NA is a homotetrameric transmembrane glycoprotein responsible for cleavage of sialic acid from the host cell membrane. By blocking NA enzymatic activity, neuraminidase inhibitors (NAIs) prevent new viral particles from being released from the surface of an infected cell, thus stopping the spread of virus in the airways. In this study, we applied a set of experimental techniques using recombinant NA variants to understand the molecular basis of development of oseltamivir resistance in the viral N1 neuraminidase NA2009. To decipher the structural mechanism of resistance, we determined crystal structures of NA2009 mutants in complex with oseltamivir carboxylate.

Two variants (I223V and S247N single mutants) crystallized in the centered orthorhombic space group with two molecules in the asymmetric unit; the tetrameric biological unit could be reconstructed from two symmetrically related dimers. The I223V substitution did not induce any structural changes in the neighboring residues; however, the substitution for a smaller side chain results in enlargement of the volume of the enzyme active site pocket and loss of Van der Waals contacts with the pentyloxy substituent of oseltamivir. The methyl group of the I223 side chain in the wt enzyme forms a dispersion bond (C-C distance of 4.1 Å) with the methyl group of oseltamivir. This interaction is not present in the I223V mutant, where the closest C-C distance between V223 and oseltamivir methyl groups is 5.0 Å. The energy of this interaction can be estimated as ~1 kcal/mol. This explains the 30-fold increase in Ki value for oseltamivir upon I to V substitution. The enthalpy change in I223V NA2009 was partly compensated by a more favorable entropic contribution of 0.6 kcal mol−1. The I223V and S247N substitutions did not have a dramatic effect on the oseltamivir binding pose. Rather, small structural alterations—such as loss of a dispersion bond with oseltamivir in the V223 mutant and changes in the hydration shell in the N247 mutant—appear responsible for increases in Ki.

>[2x]SVKLAGNSSLCPVSGWAIYSKDNSVRIGSKGDVFVIREPFISCSPLECRTFFLTQGALLNDKHSNGTIKDRSPYRTLMSCPIGEVPSPYNSRFESVAWSASACHDGINWLTIGISGPDNGAVAVLKYNGIITDTIKSWRNNVLRTQESECACVNGSCFTVMTDGPSNGQASYKIFRIEKGKIVKSVEMNAPNYHYEECSCYPDSSEITCVCRDNWHGSNRPWVSFNQNLEYQIGYICSGIFGDNPRPNDKTGSCGPVSSNGANGVKGFSFKYGNGVWIGRTKSISSRNGFEMIWDPNGWTGTDNNFSIKQDIVGINEWSGYSGSFVQHPELTGLDCIRPCFWVELIRGRPKENTIWTSGSSISFCGVNSDTVGWSWPDGAELPFTIDK> SAEKLFTPLKVGAVTAPNRVFMAPLTRLRSIEPGDIPTPLMGEYYRQRA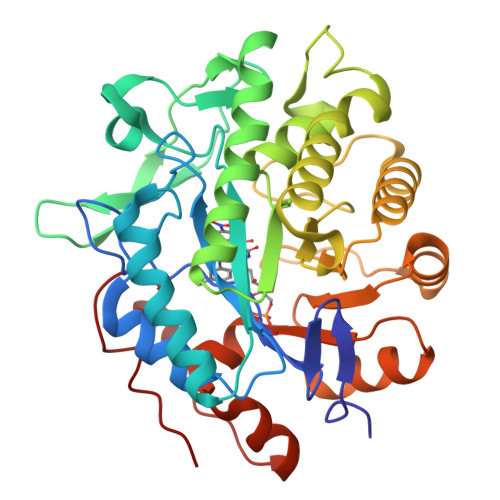SAGLIISEATQISAQAKGYAGAPGLHSPEQIAAWKKITAGVHAEDGRIAVQLFHTGRISHSSIQPGGQAPVSASALNANTRTSLRDENGNAIRVDTTTPRALELDEIPGIVNDFRQAVANAREAGFDLVELHSAHGYLLHQFLSPSSNQRTDQYGGSVENRARLVLEVVDAVCNEWSADRIGIRVSPIGTFQNVDNGPNEEADALYLIEELAKRGIAYLHMSETDLAGGKPYSEAFRQKVRERFHGVIIGAGAYTAEKAEDLIGKGLIDAVAFGRDYIANPDLVARLQKKAELNPQRPESFYGGGAEGYTDYPSL>GMRAEGLGGLERFCSPGKGRGLRALQPFQVGDLLFSCPAYAYVLTVNERGNHCEYCFTRKEGLSKCGRCKQAFYCNVECQKEDWPMHKLECSPMVVFGENWNPSETVRLTARILAKQKIHPERTPSEKLLAVKEFESHLDKLDNEKKDLIQSDIAALHHFYSKHLEFPDNDSLVVLFAQVNCNGFTIEDEELSHLGSAIFPDVALMNHSCCPNVIVTYKGTLAEVRAVQEIKPGEEVFTSYIDLLYPTEDRNDRLRDSYFFTCEC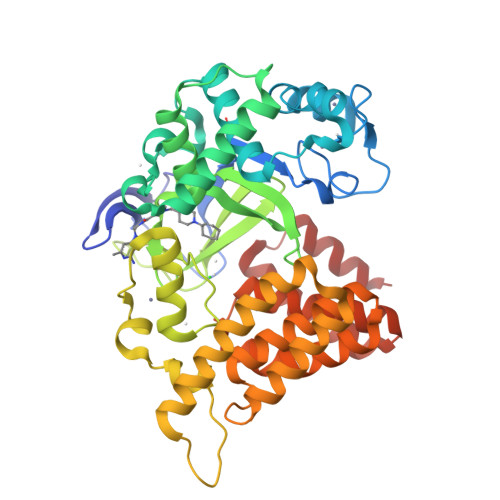QECTTKDKDKAKVEIRKLSDPPKAEAIRDMVRYARNVIEEFRRAKHYKSPSELLEICELSQEKMSSVFEDSNVYMLHMMYQAMGVCLYMQDWEGALQYGQKIIKPYSKHYPLYSLNVASMWLKLGRLYMGLEHKAAGEKALKKAIAIMEVAHGKDHPYISEIKQEIESH[2x]>[2x]MVAPLLKTLPFLAAAYAAELDLPNFSALNRRQDNSTSSSAGCSLDQTVAPGNLTLCGNATLFTTFRPKARFIAPEGWMNDPMGLYQRADGSIHAGYQSHPKHIQWGNISQGAAYSSDFTSWTDFNGSEGYKTIWPSQIYDIRGVFDGSIIKEGIDGYPTILYTSTSFGPLGATLNEAEGTETQSLAYTTDDGASWIKLGYGAGQNPVIYEWPETNLTGFRDPYVFQSPRLEALLANTTSITNATGDHFATISGGVHGDGARLFLYRQHTTGEFIKWTYLGPLVTTGYKESYGEWSGNYGINFETAGVTRLNPAGAAWDNGSDTTAVDFVTFGTEQGRADHQNHWPLWAAVDYEVRDNGSIEAVIAYSGVQDWGRSYAYASFPVEGYRQVSVGWIYEDDDNVILAKQFGYQGAFTLFRDLFVKVVENVSPSTPGLFEQASWSTKNSTDGMSVTVTTLGQRVVPETLAAYKGNSTVSTLAPVMLNESAAAYTPFSSQPTDRFYALTGSFEFGLNTTAKAGFRVLASEEEYTDIWFDPASENLTVVRTASSLIKSFGNDTELAKVKLYEIVGAESKTLNLTVFVDGSVIEIYANDEVALSTRAYPWLANSTGAGLLADGTTAGDVVGVSGLELWDGLVDAWPARPANTSQGLVWDGPTAAMYGLFAGY

Xanthophyllomyces dendrorhous β-fructofuranosidase (Xd-INV, EC 3.2.1.26) is a highly glycosylated dimeric enzyme that belongs to CAZy family GH32 and hydrolyzes sucrose and various fructooligosaccharides (FOS) and fructans releasing fructose. It also catalyzes the synthesis of short-chain FOS, in which the fructosyl moiety is transferred to the sucrose skeleton. Then, crystals from the inactivated pXd-INV-D80A enzyme were used for soaking experiments into β-D-fructose and the different polyphenols tested, to get the corresponding ternary intermediate complexes. All the polyphenolic compounds are bound by stacking their aromatic rings against Trp105, with additional hydrogen bonds from their OH groups to several residues at the active site directly or through several well-ordered water molecules that are linked to the protein.

Also, the crystals were soaked into hydroquinone in absence of fructose to investigate potential additional binding sites for this acceptor. In the HQ-soaked crystals, a tris(hydroxymethyl)aminomethane (Tris) molecule from the buffer was occupying the position of fructose found in the ternary complexes. As it is observed, a Tris molecule from the buffer and an ethylenglycol moiety from the cryoprotectant are mimicking fructose binding at the ‒1 subsite, while a second ethylenglycol molecule is bound similarly to that observed in the ternary complex crystals. On the other hand, the HQ molecule is stacking against Trp105, with one of its hydroxyls being linked to the C-terminal Leu661 carbonyl through water molecules. As it is observed, HQ and catechol are similarly located in both ternary complexes, while HQ is shifted in the fructose-free HQ-soaked crystals. This may suggest that binding of HQ can be more flexible than catechol binding, what would be consistent with the residual density observed in the ternary complex with HQ above mentioned.> LER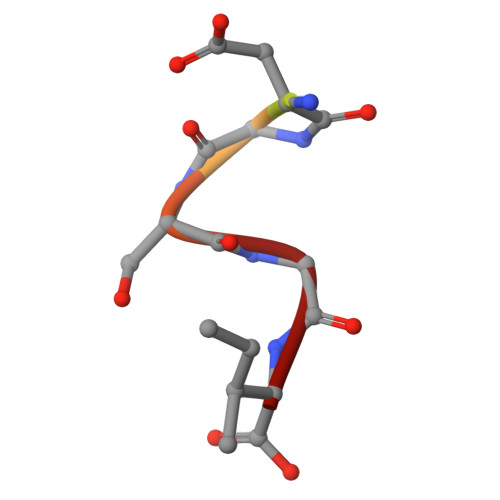DGSGI> MASAPIGSAIPRNNWAVTCDSAQSGNECNKAIDGNKDTFWHTFYGANGDPKPPHTYTIDMKTTQNVNGLSVLPRQDGNQNGWIGRHEVYLSSDGTNWGSPVASGSWFADSTTKYSNFETRPARYVRLVAITEANGQPWTSIAEINVFQASSYTAPQPGLGRWGPTIDLPIVPAAAAIEPTSGRVLMWSSYRNDAFEGSPGGITLTSSWDPSTGIVSDRTVTVTKHDMFCPGISMDGNGQIVVTGGNDAKKTSLYDSSSDSWIPGPDMQVARGXQSSATMSDGRVFTIGGSWSGGVFEKNGEVYSPSSKTWTSLPNAKVNPMLTADKQGLYRSDNHAWLFG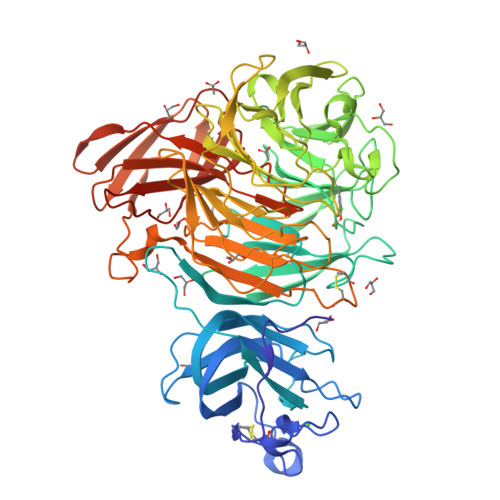WKKGSVFQAGPSTAMNWYYTSGSGDVKSAGKRQSNRGVAPDAMCGNAVMYDAVKGKILTFGGSPDYQDSDATTNAHIITLGEPGTSPNTVFASNGLYFARTFHTSVVLPDGSTFITGGQRRGIPFEDSTPVFTPEIYVPEQDTFYKQNPNSIVRAYHSISLLLPDGRVFNGGGGLCGDCTTNHFDAQIFTPNYLYDSNGNLATRPKITRTSTQSVKVGGRITISTDSSISKASLIRYGTATHTVNTDQRRIPLTLTNNGGNSYSFQVPSDSGVALPGYWMLFVMNSAGVPSVASTIRVTQLEHHHHHH> MTYKYNCCDDGSGTTVGSVVRFDNVTLLIDPGWNPSKVSYEQCIKYWEKVIPEIDVIILSQPTIECLGAHSLLYYNFTSHFISRIQVYATLPVINLGRVSTIDSYASAGVIGPYDTNKLDLEDIEISFDHIVPLKYSQLVDLRSRYDGLTLLAYNAGVCPGGSIWCISTYSEKLVYAKRWNHTRDNILNAASILDATGKPLSTLMRPSAIITTLDRFGSSQPFKK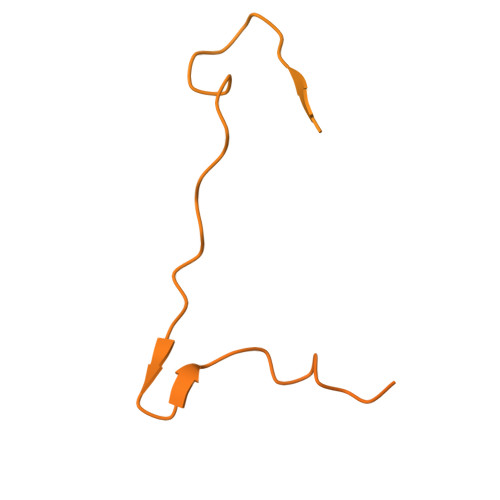RSKIFKDTLKKGLSSDGSVIIPVDMSGKFLDLFTQVHELLFESTKINAHTQVPVLILSYARGRTLTYAKSMLEWLSPSLLKTWENRNNTSPFEIGSRIKIIAPNELSKYPGSKICFVSEVGALINEVIIKVGNSEKTTLILTKPSFECASSLDKILEIVEQDERNWKTFPEDGKSFLCDNYISIDTIKEEPLSKEETEAFKVQLKEKKRDRNKKILLVKRESKKLANGNAIIDDTNGERAMRNQDILVENVNGVPPIDHIMGGDEDDDEEEENDNLLNLLKDNSEKSAAKKNTEVPVDIIIQPSAASKHKMFPFNPAKIKKDDYGTVVDFTMFLPDDSDNVNQNSRKRPLKDGAKTTSPVNEEDNKNEEEDGYNMSDPISKRSKHRASRYSGFSGTGEAENFDNLDYLKIDKTLSKRTISTVNVQLKCSVVILNLQSLVDQRSASIIWPSLKSRKIVLSAPKQIQNEEITAKLIKKNIEVVNMPLNKIVEFSTTI>MSQVGGRGDRCTQEVQGLVHGAGDLSASLAENSPTMSQNGYFEDSSYYKCDTDDTFEAREEILGDEAFDTANSSIVSGESIRFFVNVNLEMQATNTENEATSGGCVLLHTSRKYLKLKNFKEEIRAHRDLDGFLAQASIVLNETATSLDNVLRTMLRRFARDPDNNEPNCNLDLLMAMLFTDAGAPMRGKVHLLSDTIQGVTATVTGVRYQQSWLCIICTMKALQKRHVCISRLVRPQNWGENSCEVRFVILVLAPPKMKSTKTAMEVARTFATMFSDIAFRQKLLETRTEEEFKEALVHQRQLLTMVSHGPVAPRTKERSTVSLPAHRHPEPPKCKDFVPFGKGIREDIARRFPLYPLDFTDGIIGKNKAVGKYITTTLFLYFACLLPTIAFGSLNDENTDGAIDVQKTIAGQSIGGLLYALFSGQPLVILLTTAPLALYIQVIRVICDDYDLDFNSFYAWTGLWNSFFLALYAFFNLSLVMSLFKRSTEEIIALFISITFVLDAVKGTVKIFWKYYYGHYLDDYHTKRTSSLVSLSGLGASLNASLHTALNASFLASPTELPSATHSGQATAVLSLLIMLGTLWLGYTLYQFKKSPYLHPCVREILSDCALPIAVLAFSLISSHGFREIEMSKFRYNPSESPFAMAQIQSLSLRAVSGAMGLGFLLSMLFFIEQNLVAALVNAPENRLVKGTAYHWDLLLLAIINTGLSLFGLPWIHAAYPHSPLHVRALALVEERVENGHIYDTIVNVKETRLTSLGASVLVGLSLLLLPVPLQWIPKPVLYGLFLYIALTSLDGNQLVQRVALLLKEQTAYPPTHYIRRVPQRKIHYFTGLQVLQLLLLCAFGMSSLPYMKMIFPLIMIAMIPIRYILLPRIIEAKYLDVMDAEHRP[2x]

BTR1 (SLC4A11) is a NH3 stimulated H+ (OH-) transporter belonging to the SLC4 family. Dysfunction of BTR1 leads to diseases such as congenital hereditary endothelial dystrophy (CHED) and Fuchs endothelial corneal dystrophy (FECD). BTR1 shares a similar membrane topology with other SLC4 family members, with its substrate binding sites located in the central cavity between the gate and core domains. The TMD contains a core domain (comprising TMs 1–4 and 8–11) and a gate domain (comprising TMs 5–7 and 12–14), resembling the arrangement of UraA25.

To further explore how PIP2 participates in the complete substrate transport process of BTR1 and prove the connection between PIP2 and pH sensing, we attempted to solve the structures of BTR1 with the R125H mutation or wild-type BTR1 prepared under acidic pH, which may both disrupt the interaction between BTR1 and PIP2, and succeed in achieving resolutions of 2.96 Å and 2.94 Å, respectively. Intriguingly, two structures are nearly indistinguishable in conformation (RMSD = 0.250 Å), and both lack the densities of PIP2. These results suggest that the disruption of PIP2 binding site and acidic pH can both lead to the dissociation of PIP2. Non-PIP2 binding BTR1 occupies a 3D space of ~100 Å × 55 Å × 85 Å. Compared with the structures of BTR1 in the outward-facing state, the distinct features of the non-PIP2 binding BTR1 structures involve that the NTD has undergone a significant twist, as well as an apparent conformational change has taken place in the TMD. Analysis of the TMDs using HOLE2 shows that the substrate binding sites of BTR1 in these two states are accessible from the intracellular side, suggesting their inward-facing conformation. Disruption of the PIP2 binding sites (BTR1IF/R125H state) or acidic pH (BTR1IF/5.5 state) both turn BTR1 into the inward-facing conformation. Protonation of PIP2 under acidic pathological condition or pathogenic mutations exist in the L site of BTR1 lead to the disruption of the interaction between PIP2 and BTR1. Thus, we hypothesize that PIP2 molecules participate in the pH sensing process of BTR1 through passively changing their binding affinity with BTR1 under alkaline or acidic pH. Here we suggest that PIP2 may participate in sensing the intracellular pH by changing its affinity to BTR1.> MPPKVTSELLRQLRQAMRNSEYVTEPIQAYIIPSGDAHQSEYIAPCDCRRAFVSGFDGSAGTAIITEEHAAMWTDGRYFLQAAKQMDSNWTLMKMGLKDTPTQEDWLVSVLPEGSRVGVDPLIIPTDYWKKMAKVLRSAGHHLIPVKENLVDKIWTDRPERPCKPLLTLGLDYTGISWKDKVADLRLKMAERNVMWFVVTALDEIAWLFNLRGSDVEHNPVFFSYAIIGLETIMLFIDGDRIDAPSVKEHLLLDLGLEAEYRIQVHPYKSILSELKALCADLSPREKVWVSDKASYAVSETIPKDHRCCMPYTPICIAKAVKNSAESEGMRRAHIKDAVALCELFNWLEKEVPKGGVTEISAADKAEEFRRQQADFVDLSFPTISSTGPTGAIIHYAPVPETNRTLSLDEVYLIDSGAQYKDGTTDVTRTMHFETPTAYEKECFTYVLKGHIAVSAAVFPTGTKGHLLDSFARSALWDSGLDYLHGTGHGVGSFLNVHEGPCGISYKTFSDEPLEAGMIVTDEPGYYEDGAFGIRIENVVLVVPVKTKYNFNNRGSLTLEPLTLVPI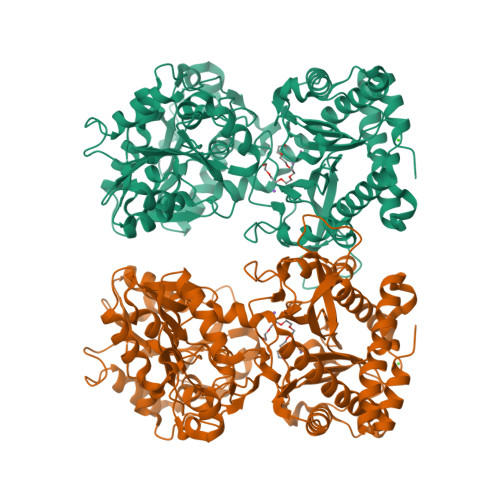QTKMIDVDSLTDKECDWLNNYHLTCRDVIGKELQKQGRQEALEWLIRETQPISKQH> MGHHHHHHMVPISPIETVPVKLKPGMDGPKVKQWPLTEEKIKALVEICTEMEKEGKISKIGPENPYNTPVFAIKKKDSTKWRKLVDFRELNKRTQDFWEVQLGIPHPAGLKQKKSVTVLDVGDAYFSVPLDKDFRKYTAFTIPSINNETPGIRYQYNVLPQGWKGSPAIFQCSMTKILEPFRKQNPDIVIYQYMDDLYVGSDLEIGQHRTKIEELRQHLLRWGFITPDKKHQKEPPFLWMGYELHPDKWTVQPIVLPEKDSWTVNDIQKLVGKLNWASQIYAGIKVRQLCKLLRGTKALTEVVPLTEEAELELAENREILKEPVHGVYYDPSKDLIAEIQKQGQGQWTYQIYQEPFKNLKTGKYARMKGAHTNDVKQLTEAVQKIATESIVIWGKTPKFKLPIQKETWEAWWTEYWQATWIPEWEFVNTPP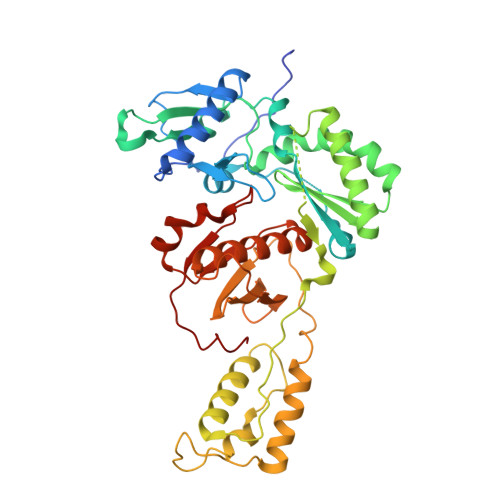LVKLWYQ>SSSSTASASAKKIIVKHVTVIGGGLMGAGIAQVAAATGHTVVLVDQTEDILAKSKKGIEESLRKVAKKKFAENPKAGDEFVEKTLSTIATSTDAASVVHSTDLVVEAIVENLKVKNELFKRLDKFAAEHTIFASNTSSLQITSIANATTRQDRFAGLHFFNPVPVMKLV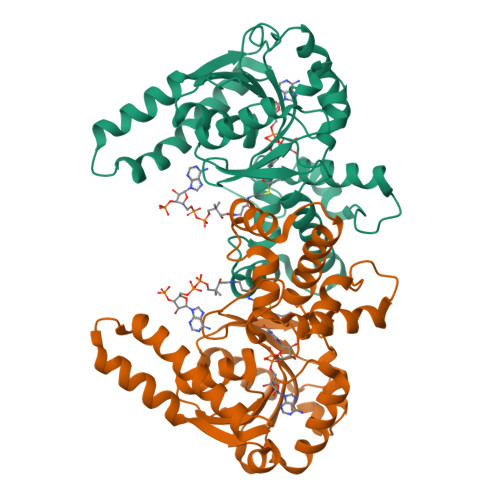EVIKTPMTSQKTFESLVDFSKALGKHPVSCKDTPGFIVSRLLVPYLMEAIRLYERGDASKEDIDTAMKLGAGYPMGPFELLDYVGLDTTKFIVDGWHEMDAENPLHQPSPSLNKLVAENKFGKKTGEGFYKYK[2x]>[2x]QVLCTNPLDIGELRSFKSKQCVDIVGNQGSGNIATYDCDGLSDQQIIICGDGTIRNEARNYCFTPDGSGNANVMSSPCTLYPEIPSSQRWRQGRRKTFTDNGGIEQVATEIINLASGKCLDIEGSDGTGDIGVYDCQNLDDQYFYVRSRGPELFYGRLRNEKSDLCLDVEGSDGKGNVLMY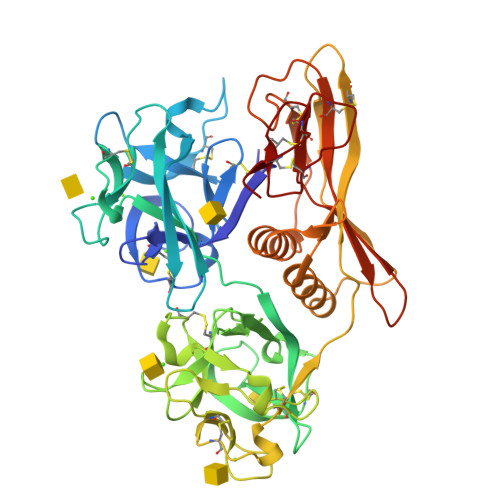SCEDNLDQWFRYYENGEIVNAKSGMCLDVEGSDGSGNVGIYRCDDLRDQMWSRPNAYCNGDYCSFLNKESNKCLDVSGDQGTGDVGTWQCDGLPDQRFKWVFDDWEVPTATWNMVGCDQNGKVSQQISNTISFSSTVTAGVAVEVSSTIEKGVIFAKATVSVKVTASLSKAWTNSQSGTTAITYTCDNYDSDEEFTRGCMWQLAIETTEVKSGDLLVWNPQIVKCTRSNTAPGCAPFTKCANEDCTFCTDI>MAAAAAEEGMEPRALQYEQTLMYGRYTQDLGAFAKEEAARIRLGGPEPWKGPPSSRAAPELLEYGRSRCARCRVCSVRCHKFLVSRVGEDWIFLVLLGLLMALVSWVMDYAIAACLQAQQWMSRGLNTSILLQYLAWVTYPVVLITFSAGFTQILAPQAVGSGIPEMKTILRGVVLKEYLTLKTFIAKVIGLTCALGSGMPLGKEGPFVHIASMCAALLSKFLSLFGGIYENESRNTEMLAAACAVGVGCCFAAPIGGVLFSIEVTSTFFAVRNYWRGFFAATFSAFIFRVLAVWNRDEETITALFKTRFRLDFPFDLQELPAFAVIGIASGFGGALFVYLNRKIVQVMRKQKTINRFLMRKRLLFPALVTLLISTLTFPPGFGQFMAGQLSQKETLVTLFDNRTWVRQGLVEELEPPSTSQAWNPPRANVFLTLVIFILMKFWMSALATTIPVPCGAFMPVFVIGAAFGRLVGESMAAWFPDGIHTDSSTYRIVPGGYAVVGAAALAGAVTHTVSTAVIVFELTGQIAHILPVMIAVILANAVAQSLQPSLYDSIIRIKKLPYLPELGWGRHQQYRVRVEDIMVRDVPHVALSCTFRDLRLALHRTKGRMLALVESPESMILLGSIERSQVVALLGAQLSPARRRQHMQERRATQTSPLSDQEGPPTPEASVCFQVNTEDSAFPAARGETHKPLKPALKRGPSVTRNLGESPTGSAESAGIALRSLFCGSPPPEAASEKLESCEKRKLKRVRISLASDADLEGEMSPEEILEWEEQQLDEPVNFSDCKIDPAPFQLVERTSLHKTHTIFSLLGVDHAYVTSIGRLIGIVTLKELRKAIEGSVTAQGVKVRPPLASFRDSATSSSDTETTEVHALWGPHSRHGLPREGSPSDSDDKCQ[2x]

CLC-2 is a voltage-gated chloride channel that contributes to electrical excitability and ion homeostasis in many different tissues. Among the nine mammalian CLC homologs, CLC-2 is uniquely activated by hyperpolarization, rather than depolarization, of the plasma membrane. The TM region of CLC-2 displays a typical CLC family symmetric homodimeric structure, with each subunit containing an independent Cl− pathway. All eukaryotic CLCs contain a pair of ‘cystathionine β-synthase’ (CBS) domains in their intracellular C-terminal domain (CTD).

While the TM domain could be resolved to 2.7 Å, the CTD exhibited poor density compared to the apo sample and did not allow us to confidently model the CTD when masking the whole protein for refinement. To improve the density quality, we masked the CTD only for refinement; this masking provided an acceptable density map at 4 Å and allowed us to confidently dock the CTD from apo structure (Figure 7—figure supplements 1–4). The orientation of the CTD in the AK-42-bound structure is the same as observed in the apo structure that shows N-terminal hairpin binding; the density for the J-K helix is weaker than in the apo dataset, but still sufficient to allow modeling of the helix.>VAKEWQENKSWNAHFTEHKSQGVVVLWNENKQQGFTNNLKRANQAFLPASTFKIPNSLIALDLGVVKDEHQVFKWDGQTRDIATWNRDHNLITAMKYSVVPVYQEFARQIGEARMSKMLHAFDYGNEDISGNVDSFWLDGGIRISATEQISFL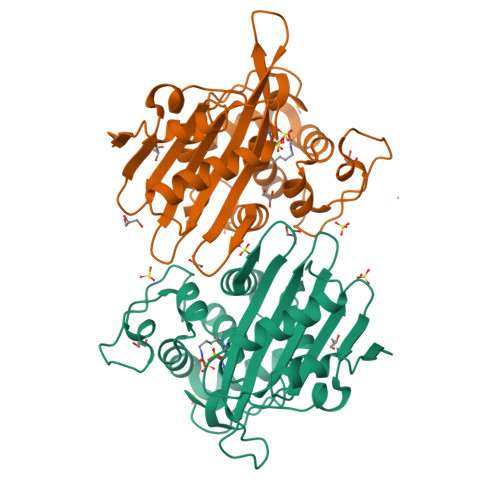RKLYHNKLHVSERSQRIVKQAMLTEANGDYIIRAKTGTGSLSDAKGGKAKIGWWVGWVELDDNVWFFAMNMDMPTSDGLGLRQAITKEVLKQEKIIPF[2x]>SQNGRIDPFTLVLGPLYAIDAPFAVNLVSQNGRRYLKASISLELSNEKLLNEVKVKDTAIKDTIIEILSSKSVEEVVTNKGK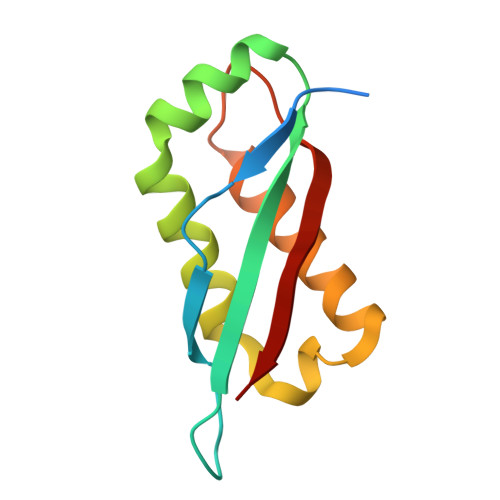NKLKDEIKSHLNSFLIDGFIKNVFFTDFIIQ[6x]>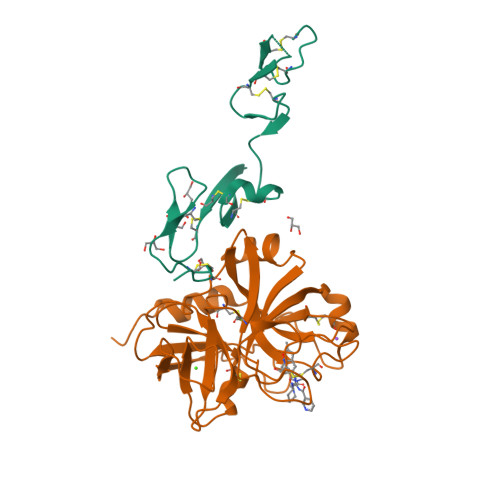KDGDQCETSPCQNQGKCKDGLGEYTCTCLEGFEGKNCELFTRKLCSLDNGDCDQFCHEEQNSVVCSCARGYTLADNGKACIPTGPYPCGKQTLE[2x];>IVGGQECKDGECPWQALLINEENEGFCGGTILSEFYILTAAHCLYQAKRFKVRVGDRNTEQEEGGEAVHEVEVVIKHNRFTKETYDFDIAVLRLKTPITFRMNVAPACLPERDWAESTLMTQKTGIVSGFGRTHEKGRQSTRLKMLEVPYVDRNSCKLSSSFIITQNMFCAGYDTKQEDACQGDSGGPHVTRFKDTYFVTGIVSWGEGCARKGKYGIYTKVTAFLKWIDRSMKTRGLP[2x]> MAAGTFTAQNKVRPGVYINFKSEPQAAGTLGERGIVSMPLILSWGEPGKMITIEAGDDVFPKLGYSIMDAQLRLINEALKRAKTLLLYRLN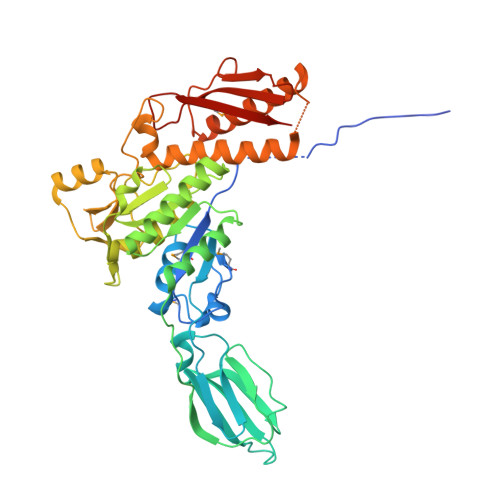AGTKAAVTVGNLTVTAKWGGARGNDITLVIQENIDDETKFDVSTLVDGAELDKQTVSDIAGLAANDWVIFSGTGALTETAGAPLINGSDGAVTNQAYIDYLAAVEIFDFNTIALPSTDDALKATFTAFAKRLRDDEGKKIQVVLENYPAADYEGVISVKNGVVLADGTILTAAQATAWVAGATAGARVNESLTYQGYDEAVDVAPRYTNAQIIAALQAGEFLFTASDNQALVEQDINTLTSFTADKGKQFAKNRVIRVLDGINNDFVRIFSKFYIGKVSNNADGRNLLKSECINYMNTLQDIDAIKNFDGQTDLTVQSGNDVDAVYIEAYAWPVDSIEKIYVRVRIKLEHHHHHH2-(furan-2-yl)ethanamine | C6 H9 N O | 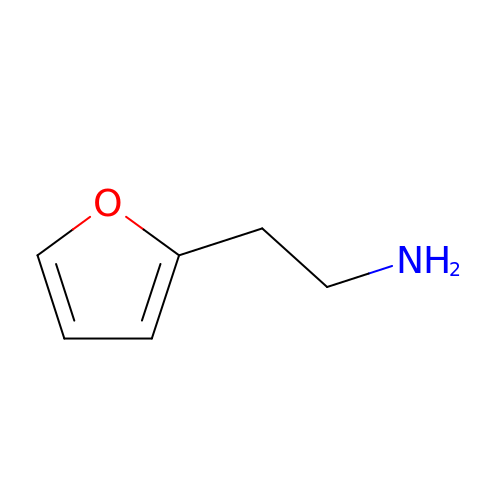ZQSLNSHMUQXSQJ-UHFFFAOYSA-N> 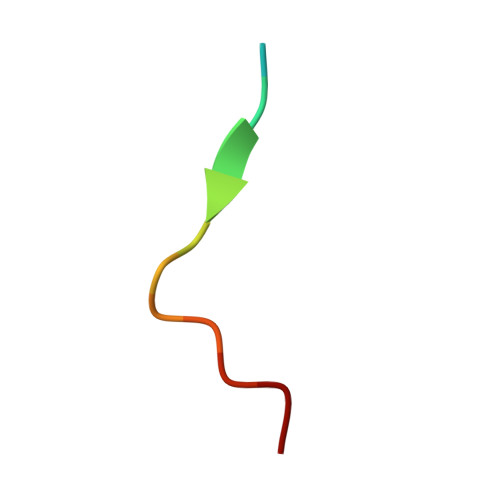XQNGFDNPNYQPQ> TMITHHHHHHGSMHYKAQLQKLLTTEEKKILARLSTPQKIQDFLDTIKNKDLAEGEHTMWSPRAVLKHKHAHCMEGAMLAALALAYHGHSPLLMDLQTTDEDEDHVVALFKIDGHWGAISKTNHPVLRYRDPIYKSVRELAMSYFHEYFIWWTKKNGGKKTLRAYSNPFDLTRYKPERWVIATGDLDWLAEALDDSKHFPILNKKMQKQLRPASRIETKAASLSEWPKRKTNS

Here, we present the structural and functional elucidation of CPR-C4, a hypothetical protein from the genome of a thermophilic Candidate Phyla Radiation organism, identified through metagenomic sequencing. The function of CPR-C4 as a cysteine protease was predicted through remote structural similarity to the Homo sapiens vasohibins and subsequently confirmed experimentally with fluorescence-based activity assays. Furthermore, detailed structural and sequence alignment analysis enabled identification of a noncanonical cysteine-histidine-leucine(carbonyl) catalytic triad. In all crystal forms, the structure of CPR-C4 is a homodimer displaying a mixed αβ fold, with a central curved antiparallel β-sheet surrounded by short α-helices connected by flexible loops.

The CPR-C4 protein, including an N-terminal His6-tag, crystallized in two space groups with different crystal morphologies but similar resolution limits. Crystal form 2 diffracted to a resolution of 2.68 Å in space group I222, with one polypeptide chain per asymmetric unit, and was solved by molecular replacement with the model from crystal form 1. Surprisingly, the two Zn2+ ions were only present in crystal form 1 and were both found to interact with the same chain (chain A), in a tetrahedral geometry, as is most common for Zn2+ coordination. However, the absence of other metal cations in the zinc-free crystal structures implies this is not a promiscuous site, and the tetrahedral ligand arrangement is strongly preferable for Zn2+ binding over other transition metal cations or the sodium and potassium present in the buffers used.>[2x]ANDTILPLNNIQGDILVGMKKQKERFVFFQVNDATSFKTALKTYVPERITSAAILISDPSQQPLAFVNLGFSNTGLQALGITDDLGDAQFPDGQFADAANLGDDLSQWVAPFTGTTIHGVFLIGSDQDDFLDQFTDDISSTFGSSITQVQALSGSARPGDQAGHEHFGFLDGISQPSVTGWETTVFPGQAVVPPGIILTGRDGDTGTRPSWALDGSFMAFRHFQQKVPEFNAYTLA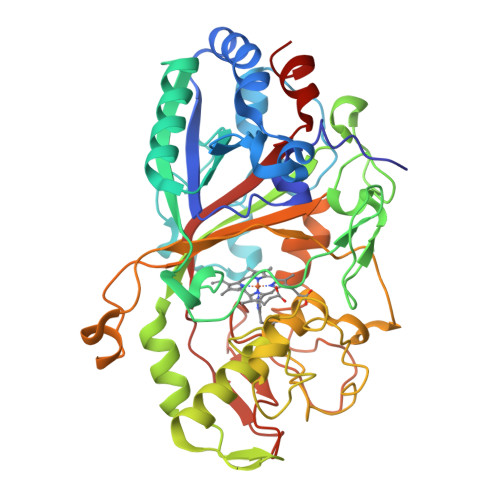NAIPANSAGNLTQQEGAEFLGARMFGRWKSGAPIDLAPTADDPALGADPQRNNNFDYSDTLTDETRCPFGAHVRKTNPRQDLGGPVDTFHAMRSSIPYGPETSDAELASGVTAQDRGLLFVEYQSIIGNGFRFQQINWANNANFPFSKPITPGIEPIIGQTTPRTVGGLDPLNQNETFTVPLFVIPKGGEYFFLPSISALTATIAA> QEGDAAKGEKEFNKCKACHMVQAPDGTDIVKGGKTGPNLYGVVGRKIASVEGF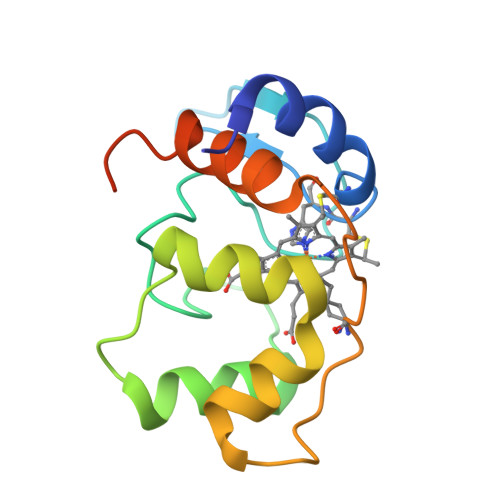KYGDGILEVAEKNPDMVWSEADLIEYVTDPKPWLVEKTGDSAAKTKKTFKLGKNQADVVAFLAQHSPDAGAEAAPAEGAAN> GPLGSEEDVPENNGILISIKEVINAEFSRDGTIHSSELKGVLELRINDHDLSHSNLKLADSIDVRDKSFQFKTHPNIDKQSFLSTKLISLRDKSKAFPANDQSLGVLRWRKVAPAEDDSLIPLTLTTAVSPSESQQGFDVIIEYESVLETELADVIFTIPVFPQEPVDINTESSTCSDAEVVNMDQEMGTSIKISKIAANDAGALAFTIEAPYEDALYPMTVSFQESTR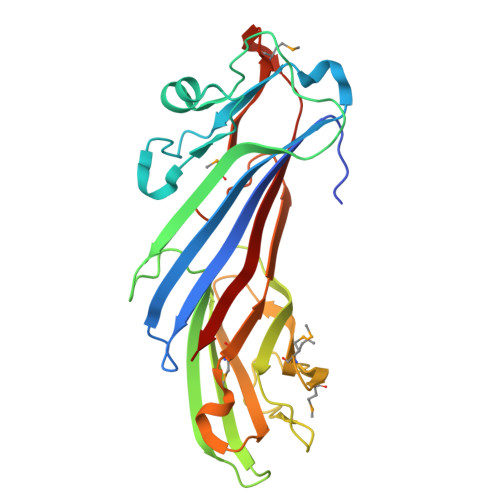DKLAKSFTGMAIQSVVMANDHDQELPYDVITSLKSDEYLVQ>MSQTLLVHGKDAQGIIKQVLSEVYDAVTSTMGPNGQLVMIKNGVSTKTTKDGVTVARSIRFADEAHELVNRVITEPATKTDEECGDGTTTTIMLTHALYHLFKDFPGFQHHRNIEDLVERVIQRLESMAIRVEVDDPRLYQVALTSSNQDEKLARLVSELYANNKGSYPDIELKEGVNFEDQIEQTTGRTIRMFYANPWFAKGHQGGVTELTGFTAFVIDRRIDKEDTQKLIDGVNHLVKTHKQHLALPILLIARSFEEAANSTLMQLNAAHPTLVEDGRPWLIPLSTPVGGAIGTSELQDIAVMLNAPMLSDVADLTKLDTHSINGQHGQLELGGNRSILKSTTPKDEDRIEQHARGI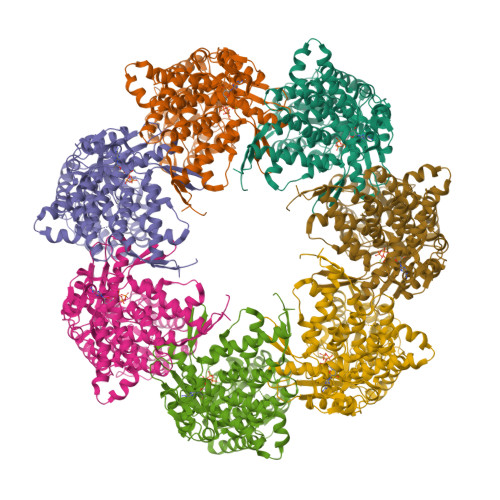EELLEGFSLSDKFSVRARYNERRIRTLRGKLITISVGGETYSEVKERVDRYEDVVKAIRSALENGILPGGGVSLVKAVFGTIKEGLEDKDQSAEFAKRYINSGIANELMRLSTIQHKLLFKDTALYKENGSFHFNDDWLNTPTVMNLATGEIGTPEGLGIYDTAYASITALKGGLQTAKILATTKTLILGEKLSAVKVR[7x]>GPGSEFEENEDSDPLPDNWEMAYTEKGEVYFIDHNTKTTSWLDPRLAKKAKPPEECK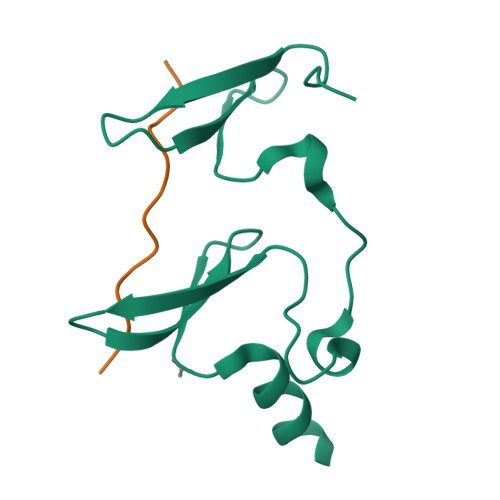ENELPYGWEKIDDPIYGTYYVDHINRRTQFENPVLEAKRKLQQHN[2x];>GPGSDRPPPYVAPPSYEG[2x]>[4x]GPMGKELKIGVPLRVSYKEFVSQIRGTENMFKGFCIDVFTAAVNL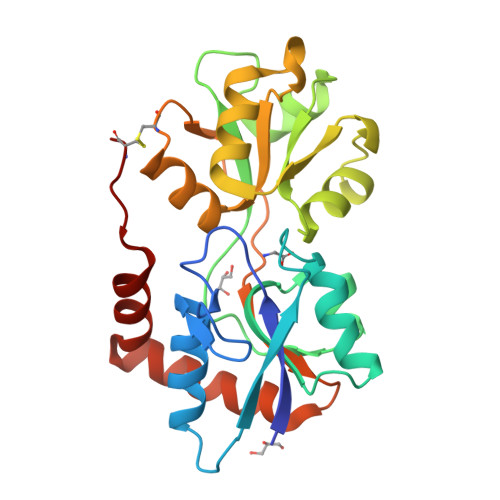LPYAVPVKFIPYGNGKENPSYTHMVEMITTGNFDGVVGDVAIVTNRTKIVDFTQPYAASGLVVVAPGGTPIKGIESLRERDDPIGYQVGSFAESYLRNELNISESRLVPLGTPEAYAKALKDGPSKGGVAAIVDERPYVELFLSSNCAYRIVGQEFTKSGWGFAFPRDSPLAIDLSTAILELAENGDLQRIHDKWLMKNACT>MVINCAFIGFGKSTTRYHLPYVLNRKDSWHVAHIFRRHAKPEEQAPIYSHIHFTSDLDEVLNDPDVKLVVVCTHADSHFEYAKRALEAGKNVLVEKPFTPTLAQAKELFALAKSKGLTVTPYQNRRFDSCFLTAKKAIESGKLGEIVEVESHFDYYRPVAETKPGLPQDGAFYGLGVHTMDQIISLFGRPDHVAYDIRSLRNKANPDDTFEAQLFYGDLKAIVKTSHLVKIDYPKFIVHGKKGSFIKYGIDQQETSLKANIMPGEPGFAADDSVGVLEYVNDEGVT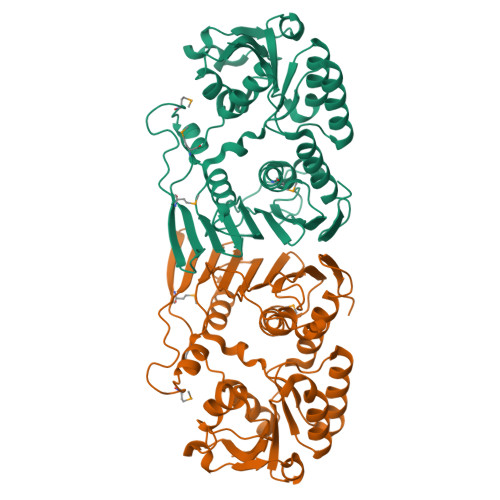VREEMKPEMGDYGRVYDALYQTITHGAPNYVKESEVLTNLEILERGFEQASPSTVTLAK[6x]> SKKRPPPPPPGH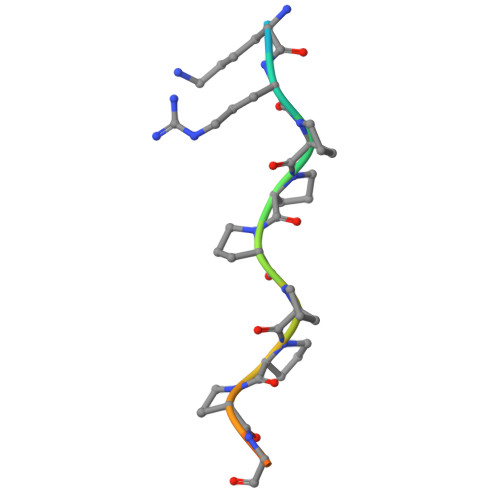KRT>MAHHHHHHMSSAESNIPEQFRIRRDKRARLLAEGYDPYPVAIERTHTLAEIRATYADLPTDSATEDIVGVAGRVVFARNTGKLCFATLQDGDGTQLQAMISLDEVGRESLDRWKADVDIGDVVYVHGTVISSRRGELSVLADSWRMAAKALRPLPVAHKEMSEESRVRQRYVDLIVRPQAREVARQRIAVIRAVRNALERRGFLEVETPMLQTLAGGAAARPFVTHSNALDIDLYLRIAPELFLKRCIVGGFDRVFELNRVFRNEGSDSTHSPEFSMLETYQTYGTYDDSALITRELIQEVADEAIGTRQLSMPDGSVYDIDGEWATMEMYSSLSEALGEQITPETTVARLRDIASGLDVEIDNSVFGHGKLVEELWEHAVGNKLTAPTFVKDFPVETTPLTRQHRSIPGVTEKWDLYVRGVELATGYSELNDPVVQRDRFADQARAAAAGDDEAMQLDEDFLTALEYGMPPCTGTGMGIDRLLMCLTGLS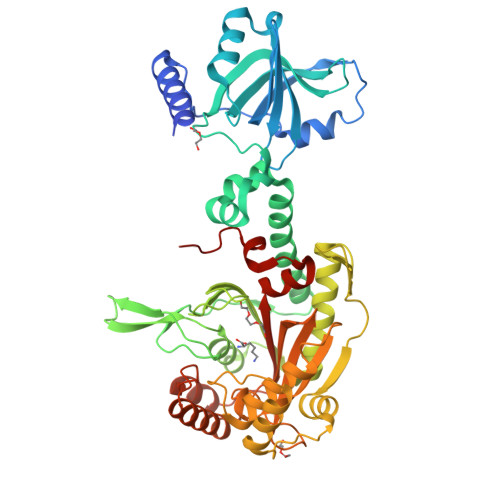IRETVLFPIVRPHSN[4x]>[4x]MIHHHHHHEHRHLKPFPPEFLWGAASAAYQVEGAWNEDGKGLSVWDVFAKQPGRTFKGTNGDVAVDHYHRYQEDVALMAEMGLKAYRFSVSWSRVFPDGNGAVNEKGLDFYDRLIEELRNHGIEPIVTLYHWDVPQALMDAYGAWESRRIIDDFDRYAVTLFQRFGDRVKYWVTLNQQNIFISFGYRLGLHPPGVKDMKRMYEANHIANLANAKVIQSFRHYVPDGKIGPS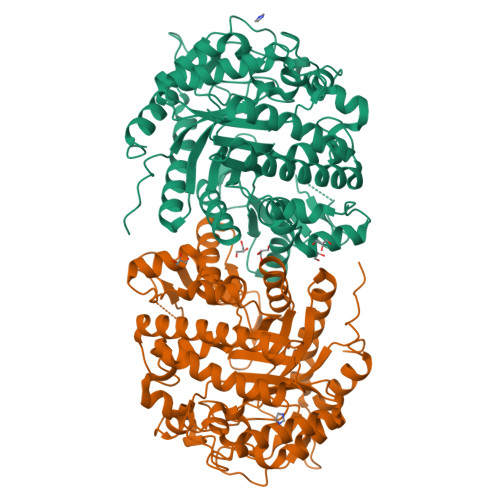FAYSPMYPYDSRPENVLAFENAEEFQNHWWMDVYAWGMYPQAAWNYLESQGLEPTVAPGDWELLQAAKPDFMGVNYYQTTTVEHNPPDGVGEGVMNTTGKKGTSTSSGIPGLFKTVRNPHVDTTNWDWAIDPVGLRIGLRRIANRYQLPILITENGLGEFDTLEPGDIVNDDYRIDYLRRHVQEIQRAITDGVDVLGYCAWSFTDLLSWLNGYQKRYGFVYVNRDDESEKDLRRIKKKSFYWYQRVIETNGAEL>[6x]MSANVDLNQRPDYDAVLQDIADYVLDYRIDSTEALDTARNCLMDTLGCGLLALRFPECTKHLGPLVEGTLVPHGARVPGTSFRLDPVKAAWDI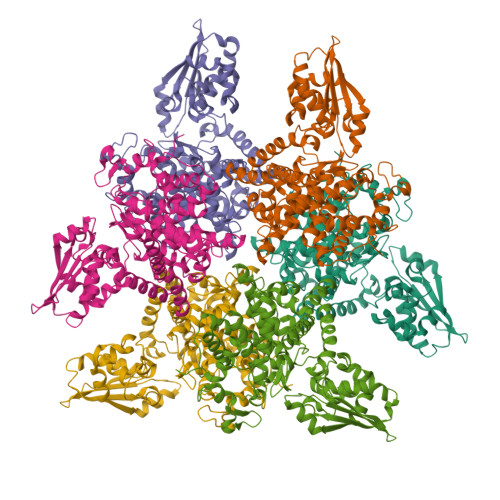GCIVRWLDYNDTWLAAEWGHPSDNLGGILAVADHLSQKRLANGEAPLSMRQVLEAMIMAHEIQGVIALENSFNRVGLDHVLLVKVASTAVCAKLMGADREQLLAALSHAFVDGQALRTYRHAPNAGSRKSWAAGDATSRGVRLADIALRGEMGIPGVLSAPQWGFYDVLFSHTSKDLATKPEDKRRFSFPQGYGSYVMENVLFKISFPAEFHAQTAAEAAVRLHPLVKDRLQRISRIVITTHESAIRIISKVGPLANPADRDHCLQYMTAVPLIFGDLVAEHYEDAFHAAHPLIDRLREKMEIVEEPRYSREYLEADKRSIANAVEVFFDDGSSTGQVAVEYPLGHRRRRAEGIPLLQEKFKANLATRFPPQRCQRIFDLCSHQASLEATPVNRFMDLLAI>[3x]AMADIGSDVASLRQQVEALQGQVQHLQAAFSQYK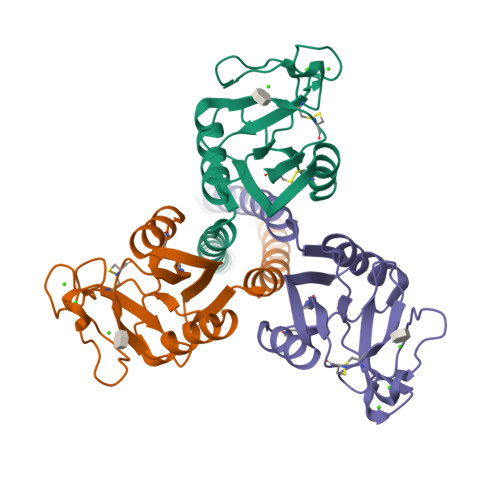KVELFPNGQSVGEKIFKTAGFVKPFTEAQLLCTQAGGQLASPRSAAENAALQQLVVAKNEAAFLSMTDSKTEGKFTYPTGESLVYSNWAPGEPNDDGGSEDCVEIFTNGKWNDRACGEKRLVVCEF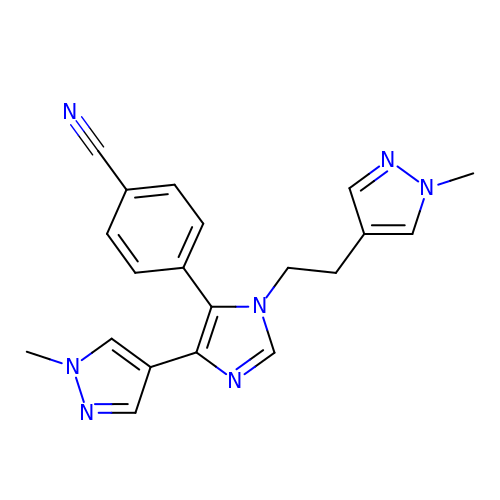4-[5-(1-methylpyrazol-4-yl)-3-[2-(1-methylpyrazol-4-yl)ethyl]imidazol-4-yl]benzenecarbonitrile | C20 H19 N7 | RRZVGDGTWNQAPW-UHFFFAOYSA-N>[4x]MGMKKSAVLN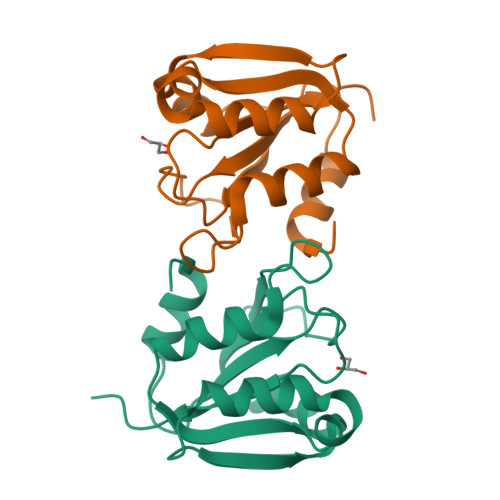EHISKAIATIGHFDLLTINDAGMPIPNDHRRIDLAVTKNLPRFIDVLATVLEEMEIQKIYLAEEIKEHNPTQLQQIKQLISSEIEIIFIPHEEMKSNLAHPLNKGNIRTGETTPYSNIALESNVTFLEHHHHHH In this study, we investigate the structure and biochemical functions of two SAPLIPs from human (Necator americanus) and dog hookworm (Ancylostoma caninum), Na-SLP-1 and Ac-SLP-1. The structure of both hookworm SAPLIPs were determined in hexagonal space groups, and closely resemble the fold of the Sap domain, as known from saposins and other SAPLIPs. The fold is comprised of a four- or five-helix bundle, where a kink in the third helix can lead to occurrence of two helices, α3 and α4. Three conserved dithioether bonds link helix α1 with the C-terminal end, helices α1 and α5, and helices α2 and α3.

Ac-SLP-1 exists exclusively as a dimer with an experimentally determined molecular mass of 19700 g/mol (MALS; theoretical M = 19062 g/mol). Despite crystallising in the same crystal system and similar cell dimensions as SLP-1 from human hookworm, the crystal structure of Ac-SLP-1 possesses only one molecule in the asymmetric unit. Ac-SLP-1, despite being a monomer in the asymmetric unit, crystallised as a P2-symmetric dimer that is aligned with one of the crystallographic axes. Buried within the dimer interface is a flat hydrophobic surface constituted mainly by the solvent-exposed side of helix α3. The buried surface area of 767 Å2 corresponds to about 30% of the monomer surface, and is thus above the threshold for specific interaction interfaces as established by Janin. The most striking feature of the Ac-SLP-1 dimer is a long linear groove connecting the large cavities at their distal ends. Near the N-terminal region, a citrate molecule was found to occupy a special position on a two-fold axis. In contrast to the human hookworm SLP-1, Ac-SLP-1 does not possess a prominent cluster of basic surface residues, but rather three small isolated basic surface areas, comprised of Lys-17/Lys-21 (α1), Lys-36 (α2) and Lys-54/Lys-57 (α3). Ac-SLP-1, in contrast, shows no such feature and has a well ordered internal side chain packing. The trigger event that leads to disassembly of the membrane-associated dimers may come from the tryptophan residue at position 48, which sits in the link area between helices α2 and α3.

> TPVVINNSNVIVCEICKMAVKLIVPEADKDLDQLEKEFIQGCMTLIGWLPYAEKECKALAKIEMGAIKTLLENGSAPEEICTTLHAC The principal constituent of the protein deposits is one of the most abundant proteins in the extracellular matrix (ECM) of the human cornea, transforming growth factor-β–induced protein (TGFBIp). The function of corneal TGFBIp is elusive, but its ability to bind both integrins and ECM molecules indicates a role in cell adhesion. TGFBIp consists of an N-terminal CROPT domain followed by four fasciclin 1 (FAS1) domains (FAS1-1, FAS1-2, FAS1-3, and FAS1-4). The X-ray crystal structure of wildtype TGFBIp reveals an elongated banana-shaped molecule with the five domains arranged like pearls on a curved string.

Among the most frequent pathogenic mutations are R124H and R555W, both associated with granular corneal dystrophy (GCD) characterized by the early-onset formation of amorphous aggregates. A striking feature found in both the R124H and R555W structures and involving their mutated residues is a crystal packing interface between the FAS1-1 and FAS1-4 domains of different TGFBIp molecules, where residue 124 interacts with residue 555 in a second TGFBIp molecule (i.e., His124 and Arg555 in R124H, Arg124 and Trp555 in R555W). In the R124H structure, the FAS1-1 His124 is in direct contact with Arg555 through a side-chain hydrogen bond. His124 also engages in a second water-bridged interaction with the main chain of Met517. The side chain of Tyr121 also forms a hydrogen bond with the main chain of Leu559 in the second TGFBIp molecule. In addition, multiple hydrophobic interactions involving side chains of Tyr121, Leu120, Met517, Phe547, Leu550, and Leu559 surround His124 and Arg555. A comparison of all available structures reveals that the R124H mutation has no influence on the structure for the FAS1-1 domain, whereas in both the R124H and the R555W structures, the α-helix harboring residue 555 is shifted relative to the position of the helix in the wildtype structure. Instead, the position of the α-helix is likely to be determined by the intermolecular contact with the FAS1-1 domain. The Arg124 and Arg555 residues in wildtype TGFBIp do not permit this intermolecular interface due to size and electrostatic repulsion between the two arginines.

> GPNVCAVQKVIGTNRKYFTNCKQWYQRKICGKSTVISYECCPGYEKVPGEKGCPAALPLSNLYETLGVVGSTTTQLYTDHTEKLRPEMEGPGSFTIFAPSNEAWASLPAEVLDSLVSNVNIELLNALRYHMVGRRVLTDELKHGMTLTSMYQNSNIQIHHYPNGIVTVNCARLLKADHHATNGVVHLIDKVISTITNNIQQIIEIEDTFETLRAAVAASGLNTMLEGNGQYTLLAPTNEAFEKIPSETLNRILGDPEALRDLLNNHILKSAMCAEAIVAGLSVETLEGTTLEVGCSGDMLTINGKAIISNKDILATNGVIHYIDELLIPDSAKTLFELAAESDVSTAIDLFRQAGLGNHLSGSERLTLLAPLNSVFKDGTPPIDAHTRNLLRNHIIKDQLASKYLYHGQTLETLGGKKLRVFVYRNSLCIENSCIAAHDKRGRYGTLFTMDRVLTPPMGTVMDVLKGDNRFSMLVAAIQSAGLTETLNREGVYTVFAPTNEAFRALPPRERSRLLGDAKELANILKYHIGDEILVSGGIGALVRLKSLQGDKLEVSLKNNVVSVNKEPVAEPDIMATNGVVHVITNVLHHHHHH> AEEWYFGKITRRESERLLLNPENPRGTFLVRESET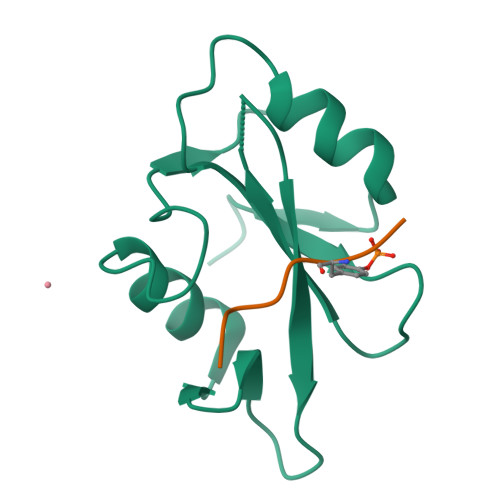TKGAYCLSVSAFANAKGLNVAHYKIRKLDSGGFYITSRTQFSSLQQLVAYYSKHADGLCHRLTNVCPT;> PQYEEIPI> KITKAMEMVAASKMRKSQDRMAASRPYAETMRKVIGHLAHGNLEYKHPYLEDRDVKRVGYLVVSTDRGLCGGLNINLFKKLLAEMKTWTDKGVQCDLAMIGSKGVSFFNSVGGNVVAQVTGMGDNPSLSELIGPVKVMLQAYDEGRLDKLYIVSNKFINTMSQVPTI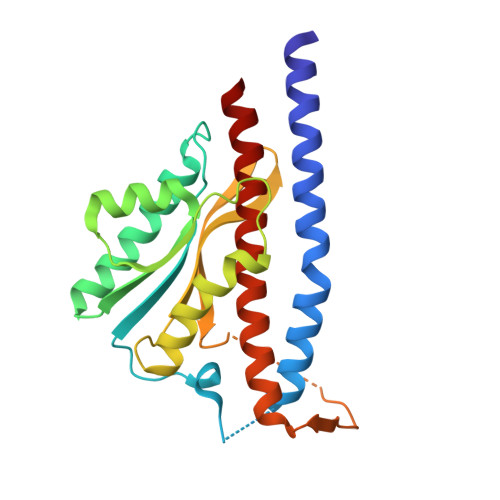SQLLPLPASDDDDLKHKSWDYLYEPDPKALLDTLLRRYVESQVYQGVVENLASEQAARMVAMK> VASVSKRIMHNAYYYDKDAKRVGTDSVKRYNSVSVLPNTTTINGKTYYQVVENGKAVDKYINAANIDGTKRTLKHNAYVYASSKKRANKVVLKKGEVVTTYG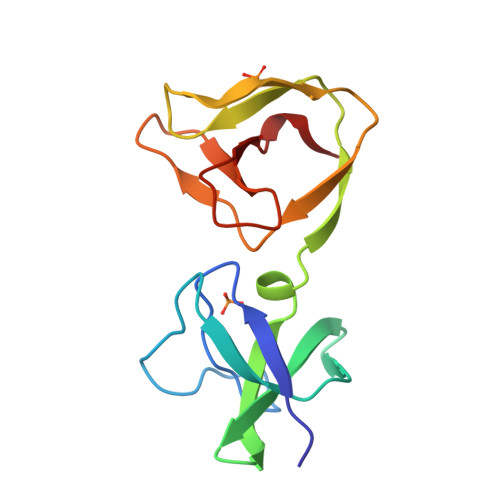ASYTFKNGQKYYKIGDNTDKTYVKVANFR(1R,2R,3S,4R,6S)-4,6-diamino-2,3-dihydroxycyclohexyl 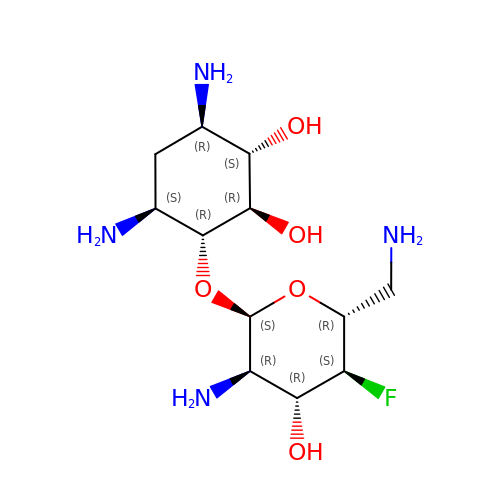2,6-diamino-2,4,6-trideoxy-4-fluoro-alpha-D-glucopyranoside | C12 H25 F N4 O5 | CRXNRBKQEXVRGM-ITWNYXCASA-N>MGHHHHHHMVLMTKPGTSDFVWNGIPLSMELNLWNIKEYSGSVAMKFDGEKITFDADIQNLSPKEPERYVLGYPEFYYGYKPWENHTAEGSKLPVPVSSMKSFSVEVSFDIHHEPSLPLNFAMETWLTREKYQTEASIGDVEIMVWFYFNNLTPGGEKIEEFTIPFVLNGESVEGTWELWLAEWGWDYLAFRLKDPVKKGRVKFDVRHFLDAAGKALSSSARV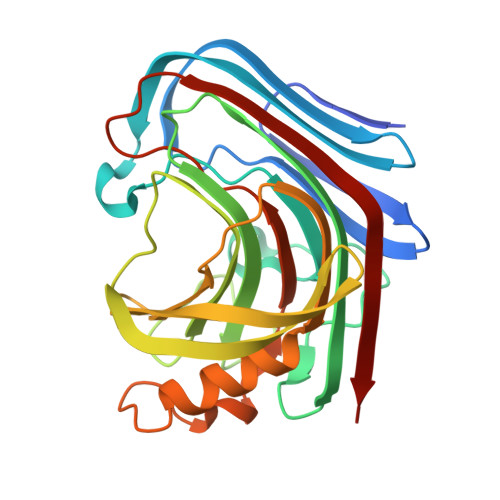KDFEDLYFTVWEIGTEFGSPETKSAQFGWKFENFSIDLEVRE[2x]> QKDANFASGRNSIVHLFEWKWNDIADECERFLQPQGFGGVQISPPNEYLVADGRPWWERYQPVSYIINTRSGDESAFTDMTRRCNDAGVRIYVDAVINHMTGMNGVGTSGSSADHDGMNYPAVPYGSGDFHSPCEVNNYQDADNVRNCELVGLRDLNQGSDYVRGV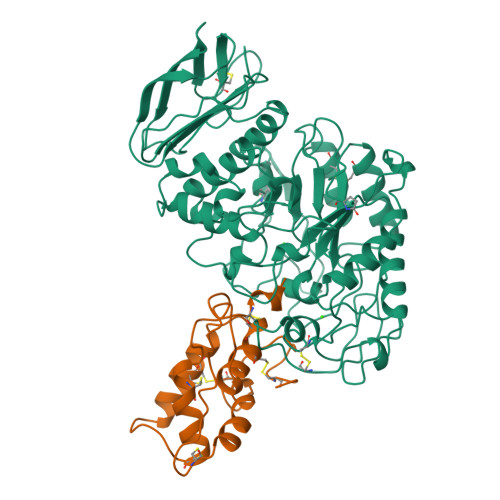LIDYMNHMIDLGVAGFRVDAAKHMSPGDLSVIFSGLKNLNTDYGFADGARPFIYQEVIDLGGEAISKNEYTGFGCVLEFQFGVSLGNAFQGGNQLKNLANWGPEWGLLEGLDAVVFVDNHDNQRTGGSQILTYKNPKPYKMAIAFMLAHPYGTTRIMSSFDFTDNDQGPPQDGSGNLISPGINDDNTCSNGYVCEHRWRQVYGMVGFRNAVEGTQVENWWSNDDNQIAFSRGSQGFVAFTNGGDLNQNLNTGLPAGTYCDVISGELSGGSCTGKSVTVGDNGSADISLGSAEDDGVLAIHVNAKL;> SVGTSCIPGMAIPHNPLDSCRWYVSTRTCGVGPRLATQEMKARCCRQLEAIPAYCRCEAVRILMDGVVTSSGQHEGRLLQDLPGCPRQVQRAFAPKLVTEVECNLATIHGGPFCLSL>[7x]MGTTTVGLVCKDGVVMATEKRATMGNFIASKAAKKIYQIADRMAMTTAGSVGDAQFLARIIKIEANLYEIRRERKPTVRAIATLTSNLLNSYRYFPYLVQLLIGGIDSEGKSIYSIDPIGGAIEEKDIVATGSGSLTAYGVLEDRFTPEIGVDEAVELAVRAIYSAMKRDSASGDGIDVVKITEDEFYQYSPEEVEQILAKFRKHHHHHH;>[7x]MGHLPQMGYDRAITVFSPDGRLFQVEYAREAVKRGATAIGIKCKEGVILIADKRVGSKLLEADTIEKIYKIDEHICAATSGLVADARVLIDRARIEAQINRLTYDEPITVKELAKKICDFKQQYTQYGGVRPFGVSLLIAGVDEVPKLYETDPSGALLEYKATAIGMGRNAVTEFFEKEYRDDLSFDDAMVLGLVAMGLSIESELVPENIEVGYVKVDDRTFKEVSPEELKPYVERANERIRELLKK;>GHMGGDSEIQYLLEKLKKLEEDYYKLRELYRRLED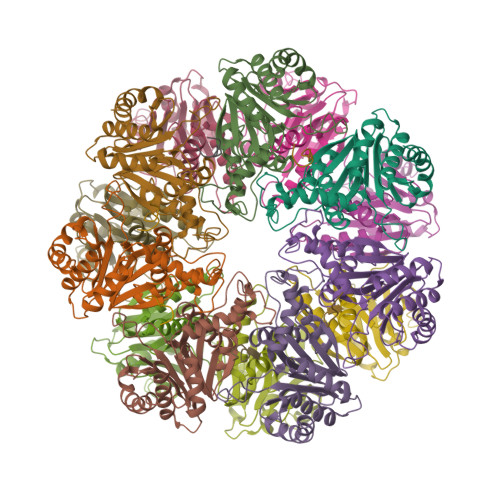EKKFIESERIRYEREVRRLRSEVERLRSPPLLVGVVSDILEDGRVVVKSSTGPKFVVNTSQYINEEELKPGARVALNQQTLAIVNVLPTSKDPMVYGFEVEEKPEVSYEDIGGLDVQIEEIREAVELPLLKPELFAEVGIEPPKGVLLYGPPGTGKTLLAKAVANQTRATFIRVVGSEFVQKYIGEGARLVREVFQLAKEKAPSIIFIDELDAIAARRTNSDTSGDREVQRTMMQLLAELDGFDPRGDVKVIGATNRIDILDPAILRPGRFDRIIEVPLPTFEGRIQIFKIHTRKMKLAEDVDFKELARITEGASGADIKAICTEAGMFAIREERAKVTMLDFTKAIEKVLKKTTPIPDLKGVMFV[6x]>[4x]SNAMTRYALLVRGINVGGKNKVVMAELRQELTNLGLEKVESYINSGNIFFTSI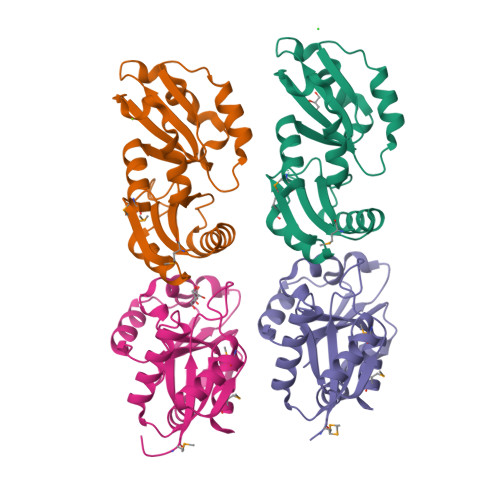DSKAQLVEKLETFFAVHYPFIQSFSLLSLEDFEAELENLPAWWSRDLARKDFLFYTEGLDVDQVIATVESLELKDEVLYFGKLGIFWGKFSEESYSKTAYHKYLLKVPFYRHITIRNAKTFDKIGQMLKK Chondroitin sulfates (CS) are linear, negatively charged, and complex polysaccharide chains ubiquitously expressed on the cell surface and within the extracellular matrix of almost all higher eukaryotes. The polysaccharide backbone consists of repeating disaccharide units of N-acetyl-D-galactosamine (GalNAc) and D-glucuronic acid (GlcA), and carries sulfate groups at various positions. Here, we identify four heterodimeric complexes responsible for chondroitin sulfate chain polymerization in humans: CHSY1-CHPF, CHSY1-CHPF2, CHSY3-CHPF, and CHSY3-CHPF2. The architecture of the catalytic sites suggests that CHSY1 and CHSY3 are enzymatically active, while CHPF and CHPF2 primarily play a stabilizing role.

The CHSY3-CHPF complex was selected for structural and functional studies due to its highest thermal stability and in vitro chain polymerization activity in our setup. An octasaccharide, (GalNAc-GlcA), representing both an acceptor substrate for the GalNAc-T reaction and the product of the GlcA-T reaction, was added to the sample, along with the donor substrate analog/reaction product UDP, prior to EM grid preparation. Cryo-EM analysis provided a 3D reconstruction at an estimated nominal resolution of 3.0 Å, revealing the overall architecture of the CS polymerase complex with its four GT domains. Predicted C-terminal α-helices of both proteins were not visible in the cryo-EM map, probably due to a high conformational flexibility. The analysis revealed that CHSY3 and CHPF form a tightly packed complex, with their respective N-terminal and C-terminal GT domains interacting strongly, resulting in a total interaction surface of 6711 Å2, as determined using PDBePISA36. Additionally, EM densities corresponding to three N-glycans were identified at asparagine residues N279 and N710 in CHSY3, and N138 in CHPF, with a fourth potential site at N361 in CHPF. Furthermore, EM density was observed for a UDP molecule and an Mn2+ ion in the active site of the N-terminal GT domain of CHSY3, as well as for an Mn2+ ion in the C-terminal GT domain of CHSY3. No EM density was observed for the octasaccharide substrate that was added during sample preparation. The active site architecture highlights key residues involved in catalyzing CS chain elongation. These include a DxD motif (D261 and D263), commonly found in GT-A fold enzymes, which, together with H394, coordinates the Mn2+ ion. Additional residues contributing to donor substrate binding in CHSY3 are D231 and K238, located near the uracil moiety; D262, which interacts with the ribose group; and R187, Y233, and K397, which stabilize the pyrophosphate group.

> GPGGSTGGENWEPRVLPYHPAQPGQAAKKAVRTRYISTELGIRQRLLVAVLTSQTTLPTLGVAVNRTLGHRLERVVFLTGARGRRAPPGMAVVTLGEERPIGHLHLALRHLLEQHGDDFDWFFLVPDTTYTEAHGLARLTGHLSLASAAHLYLGRPQDFIGGEPTPGRYCHGGFGVLLSRMLLQQLRPHLEGCRNDIVSARPDEWLGRCILDATGVGCTGDHEGVHYSHLELSPGEPVQEGDPHFRSALTAHPVRDPVHMYQLHKAFARAELERTYQEIQELQWEIQNTSHLAVDGDQAAAWPVGIPAPSRPASRFEVLRWDYFTEQHAFSCADGSPRCPLRGADRADVADVLGTALEELNRRYHPALRLQKQQLVNGYRRFDPARGMEYTLDLQLEALTPQGGRRPLTRRVQLLRPLSRVEILPVPYVTEASRLTVLLPLAAAERDLAPGFLEAFATAALEPGDAAAALTLLLLYEPRQAQRVAHADVFAPVKAHVAELERRFPGARVPWLSVQTAAPSPLRLMDLLSKKHPLDTLFLLAGPDTVLTPDFLNRCRMHAISGWQAFFPMHFQAFHPAVAPPQGPGPPELGRDTGRFDRQAASEACFYNSDYVAARGRLAAASEQEEELLESLDVYELFLHFSSLHVLRAVEPALLQRYRAQTCSARLSEDLYHRCLQSVLEGLGSRTQLAMLLFEQEQGNSTGTLEVLFQ;> GPGGSTGSGDGGAAAPSARPRDFLYVGVMTAQKYLGSRALAAQRTWARFIPGRVEFFSSQQPPNAGQPPPPLPVIALPGVDDSYPPQKKSFMMIKYMHDHYLDKYEWFMRADDDVYIKGDKLEEFLRSLNSSKPLYLGQTGLGNIEELGKLGLEPGENFCMGGPGMIFSREVLRRMVPHIGECLREMYTTHEDVEVGRCVRRFGGTQCVWSYEMQQLFHENYEHNRKGYIQDLHNSKIHAAITLHPNKRPAYQYRLHNYMLSRKISELRYRTIQLHRESALMSKLSNTEVSKEDQQLGVIPSFNHFQPRERNEVIEWEFLTGKLLYSAAENQPPRQSLSSILRTALDDTVLQVMEMINENAKSRGRLIDFKEIQYGYRRVNPMHGVEYILDLLLLYKRHKGRKLTVPVRRHAYLQQLFSKPFFRETEELDVNSLVESINSETQSFSFISNSLKILSSFQGAKEMGGHNEKKVHILVPLIGRYDIFLRFMENFENMCLIPKQNVKLVIILFSRDSGQDSSKHIELIKGYQNKYPKAEMTLIPMKGEFSRGLGLEMASAQFDNDTLLLFCDVDLIFREDFLQRCRDNTIQGQQVYYPIIFSQYDPKVTNGGNPPTDDYFIFSKKTGFWRDYGYGITCIYKSDLLGAGGFDTSIQGWGLEDVDLYNKVILSGLRPFRSQEVGVVHIFHPVHCDPNLDPKQYKMCLGSKASTFASTMQLAELWLEKHLGVRYNRTLSGTGSGLNDIFEAQKIEWHEG> VLSDFQEAVPTVVGIPDGTAVVGRSFRVSIPTDLIASSGEIIKVSAAGKEALPSWLHWNPHSHILEGLPLDTDKGVHYISVSAARLGANGSHVPQTSSVFSIEVYPEDHNEPQSVRAASSDPGEVVPSACAADEPVTVLTVILDADLTKMTP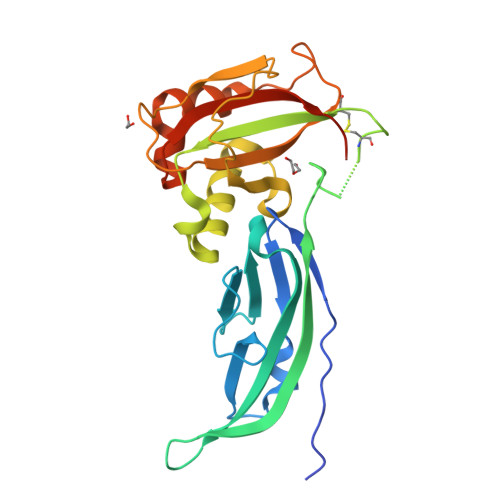KQRIDLLNRMQSFSEVELHNMKLVPVVNNRLFDMSAFMAGPGNAKKVVENGALLSWKLGCSLNQNSVPDIRGVETPAREGAMSAQLGYPVVGWHIANKKPTLPKRLRRQIH>[2x]MSVLNTPNHYKMDNSGRRVVIDPVTRIEGHMRCEVNVDENNVIQNAVSTGTMWRGLEVILRGRDPRDAWAFVERICGVCTGCHALASVRAVEDALDIKIPHNATLIREIMAKTLQIHDHIVHFYHLHALDWVNPVNALKADPQATSELQKLVSPHHPMSSPGYFKDIQIRIQKFVDSGQLGIFKNGYWSNPAYKLSPEADLMAVTHYLEALDFQKEIVKIHAIFGGKNPHPNYMVGGVPCAINIDGDMAAGAPINMERLNFVKSLIEQGRTFNTNVYVPDVIAIAAFYRDWLYGGGLSATNVMDYGAYPKTPYDKSTDQLPGGAIINGDWGKIHPVDPRDPEQVQEFVTHSWYKYPDETKGLHPWDGITEPNYELGSKTKGSRTNIIEIDESAKYSWIKSPRWRGHAVEVGPLARYILAYAQGVEYV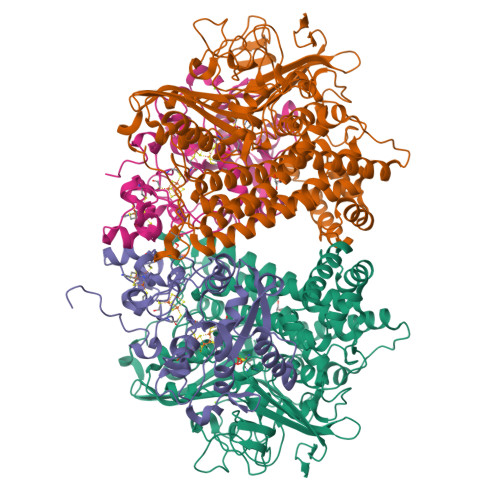KTQVHTSLNRFNAVCRLLDPNHKDITDLKAFLGSTIGRTLARALESEYCGDMMLDDFNQLISNIKNGDSSTANTDKWDPSSWPEHAKGVGTVAAPRGALAHWIVIEKGKIKNYQCVVPTTWNGSPRDPKGNIGAFEASLMGTPMERPDEPVEVLRTLHSFDPCLACSTH;>[2x]NKIAHAMETKPRTPVIWLHGLECTCCSESFIRSAHPLAKDVVLSMISLDYDDTLMAASGHAAEAILDEIKEKYKGNYILAVEGNPPLNQDGMSCIIGGRPFSEQLKRMADDAKAIISWGSCASWGCVQAAKPNPTQATPVHKFLGGGYDKPIIKVPGCPPIAEVMTGVITYMLTFDRIPELDRQGRPKMFYSQRIHDKCYRRPHFDAGQFVEEWDDEGARKGYCLYKVGCKGPTTYNACSTVRWNGGTSFPIQSGHGCIGCSEDGFWDKGSFYSRDTEMNAFG> KKP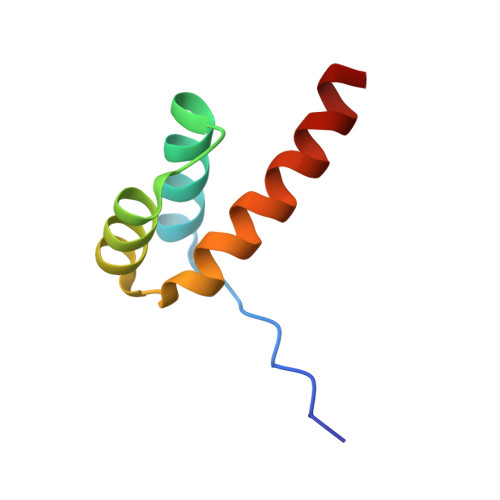RKARTAFSDHQLNQLERSFERQKYLSVQDRMDLAAALNLTDTQVKTWYQNRRTKWKRQTA>[2x]TGSTGSTGSTGSQQKRAFEYEIRFYTGNDPLDVWDRYISWTEQNYPQGGKESNMSTLLERAVEALQGEKRYYSDPRFLNLWLKLGRLCNEPLDMYSYLHNQGIGVSLAQFYISWAEEYEARENFRKADAIFQEGIQQKAEPLERLQSQHRQFQARVSRQTLLALEKEEEEEVFESS;>GPLGSSSENKIDFNDFIKRLKTGK[2x]

The multidomain protein kinase BUBR1 and its paralog BUB1 are central components of the SAC. BUBR1 also associates with unattached/incorrectly attached kinetochores and plays an important role in kinetochore microtubule interactions. Blinkin is a central component of the KNL1/Mis12/Ndc80 complexes (KMN) network, the multiprotein macromolecular assembly essential for the establishment of proper kinetochore-microtubule attachments. The interaction of Blinkin with BUB1 and BUBR1 connects SAC signaling with the KMN network and is essential for the recruitment of both multitask kinases to the kinetochore (revised in Bolanos-Garcia and Blundell, 2011).

We crystallized and solved the structure of human BUBR1 at 2.2 Å resolution in complex with Blinkin peptide in the form of the chimeric protein. Although we had previously been able to obtain a structure of free BUBR1 (D'Arcy et al., 2010), the peptide-bound complex proved recalcitrant to crystallization trials. However, the aforementioned biochemical and biophysical characterization of the BUBR1-Blinkin interaction provided a rational basis to design a chimera construct, which comprised Blinkin residues S208-K226 linked to N terminus BUBR1 via a poly(TGS) linker. A comparison of the crystal structure of BUBR1 in the ligand free form (D'Arcy et al., 2010) and in the complex shows that BUBR1 undergoes little conformational change upon binding Blinkin and preserves the features characteristic of TPR motifs, including a concave inner surface and a subtle right-handed super-helical twist of the entire structure. Electron density of the Blinkin residues N211-G225 was clearly visible and unequivocally shows that the side chains of Blinkin residues I213, F215, F218, and I219 form part of a short α helix defined by residues F215-T224 that runs parallel to the long axis of BUBR1 TPR1 and TPR2. Remarkably, the BUBR1-Blinkin structure revealed an unanticipated protein-protein interface in which Blinkin interacts with a shallow hydrophobic groove located in the convex side of the BUBR1 helical bundle. The structure indeed reveals that the interaction of Blinkin208-226 with BUBR157-220 is derived from complementary hydrophobic interfaces implicating Blinkin residues I213, F215, F218, I219, and L222. Polar contacts contribute to stabilize the BUBR157-220-Blinkin208-226 complex: salt bridges are formed between Blinkin residue R221 and BUBR1 residues E103 and E107 while hydrogen bonds are established between BUBR1 L131, a residue that is located in α helix A of TPR2, with Blinkin residue I213. However, the structure reveals that this Blinkin region undergoes a dramatic disorder-to-order transition upon BUBR1 binding, a feature also observed in TFE-titration experiments of Blinkin mimic peptides monitored by circular dichroism. The micromolar binding affinity of Blinkin S208-K226 peptide for BUBR157-220 (9.3 μM ± 0.4 in 1:1 stoichiometry) reflects a relatively moderate interaction.> GSHMMITMDDIIREGNPTLREVAKEVSLPLSEEDISLGKEMLEFLKNSQDPIKAEELHLRGGV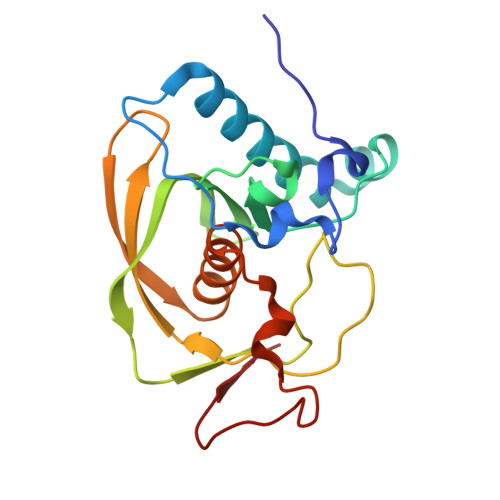GLAAPQLDISKRIIAVHVPSPDPEADGPSLSTVMYNPKILSHSVQDACLGEGEGCLSVDREVPGYVVRHAKITVSYYDMNGEKHKIRLKNYESIVVQHEIDHINGVMFYDHINDQNPFALKEGVLVIE> KVKVL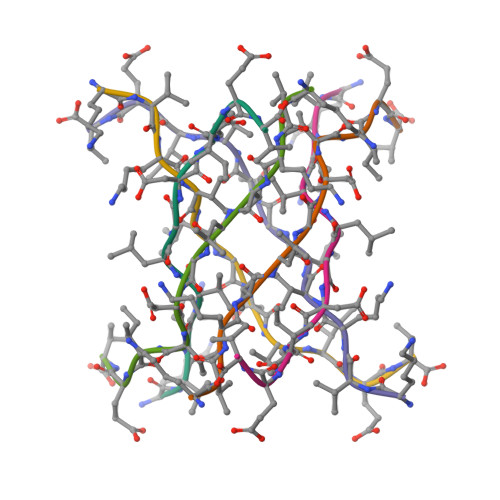GDVIEV Several natural systems exhibit ‘facilitated dissociation’, in which an effector (E) can bind to a target–host (TH) complex to form an excited ternary complex (THE)20–26 from which the target dissociates quickly. We set out to design protein systems that undergo facilitated dissociation. We use a switchable target binder (host) and a flexible effector that can rapidly bind to and switch the target–host complex to induce a large steric clash with the target, forming a strained excited ternary complex. We show here that by explicitly considering excited intermediate states when designing coupled protein systems, a broad range of facilitated dissociation systems can be designed.

To investigate the mechanism of facilitated dissociation, we focused on AS1, the design with the tightest effector binding (Kd,H:E ≈ 10 pM). We used X-ray crystallography to structurally characterize multiple states of our designed systems. For both the AS1 and the AS5 systems, the crystal structures of the hosts alone and of the host–effector complexes closely match the design models (maximum 1.3 Å Cα root mean square deviation (RMSD)). The unbound structures show an open hydrophobic cleft in the new designed state X poised to bind the effector, and the effector-bound structures show that binding the effector causes the two switch domains to register-shift into the designed state Y. The two effectors make nearly identical interactions with AS1, but when unbound, the peptide is disordered whereas the 3hb is structured. Crystal structures throughout the facilitated dissociation process confirm our ability to design excited states and large register-shift conformational changes.

>MSGSMKEEIKRLAEELKEKTKNEEIKRLAEEAAELAERSDDPEVLEVVKKALEEALKSKNEEKIELLLLVAVLVAEAGSVDAVEEKLEIALLALKLAEESKDPRIIRGALRAAIAALRSDDPLALKTVKEALERARASKDERLIRAILAAAYAFALLAVAGASAERLKEAEAIVKELIAAAEKGASPQELVLLVIEMMVKGMGVTMETHRSGNEVKVVIKGLHESQQEVLLEAVLFAAELMGVRVRIRFKGDTVTIVVRE[2x];>[2x]EERKKELAKEVIETAKKLIEKLAKEE Membrane-bound pyrophosphatases (M-PPases) are homodimeric primary ion pumps that couple the transport of Na+- and/or H+ across membranes to the hydrolysis of pyrophosphate. M-PPases are large (66–89 kDa), single-domain integral membrane proteins comprised of two identical monomers, each with 15–17 transmembrane helices. The helices of each subunit arrange into an inner ring (helices 5, 6, 11, 12, 15, 16) containing the functional core (active site, coupling funnel, ion gate, exit channel) and an outer ring (helices 1–4, 7–10, 13, 14) of largely unknown function. To date, H+-pumping (H+-PPase), Na+-pumping (Na+-PPase) and dual-pumping (Na+,H+-PPase) M-PPases have been found, most of which require potassium (K+) for maximal catalytic activity.

Following the inspection of enzyme key regions and structural alignments, it became clear that all of the data from 0 to 60 s could be combined into one, yielding a grouped structure of TmPPase in the resting state that is essentially identical to the individual 0-s (r.m.s.d./Cα: 0.33 Å) and TmPPase:CaMg (r.m.s.d./Cα: 0.29 Å) structure. The structure was solved at 2.54 Å along h, 2.95 Å along k and 3.38 Å along l with improved B-factors (108.65–70.28 Å2) and Rwork/Rfree values (21.95/23.61%) as compared to the 0-s structure (23.81/27.40%). The improvement in data quality parameters also translated into better electron density maps, so we could model most side chains and build additional key loop regions, for example, loop. Despite the presence of PPi in the crystallisation condition, it was not located at the active site, nor did it bind anywhere else. There were no observable significant changes in other regions of the protein, but the semi-conserved glutamate E6.53 appears to be flexible in all the structures as indicated by the absence of 2mFo-dFc density, even in the high-resolution 0–60 s structure, or negative density when modelled as seen in TmPPase:CaMg (Fig. EV3C). Ion binding is the first event, as there is no evidence of PPi in any of the structures before 60 s post Na+-addition, nor in the grouped 0–60-s structure, and the ion gate E6.53 appears disordered (Fig. EV3B): Na+ binding precedes substrate binding. Our TmPPase structure obtained in the absence of Na+ (0–60-s structure) suggests that in low Na+ conditions, E6.53 is not tightly coordinated at the ion gate, allowing it to loosely interact with S5.43. This could thus explain why K+-dependent Na+-PPases can pump protons at Na+ concentrations <5 mM.

>[2x]MRGSHHHHHHYVAALFFLIPLVALGFAAANFAAVVRKPEGTERMKEISSYIRSGADSFLAHETKAIFKVAIVIAILLMIFTTWQTGVAFLLGAVMSASAGIVGMKMATRANVRVAEAARTTKKIGPALKVAYQGGSVMGLSVGGFALLGLVLVYLIFGKWMGQVDNLNIYTNWLGINFVPFAMTVSGYALGCSIIAMFDRVGGGVYTKAADMAADLVGKTELNLPEDDPRNPATIADNVGDNVGDVAGLGADLLESFVGAIVSSIILASYMFPIYVQKIGENLVHQVPKETIQALISYPIFFALVGLGCSMLGILYVIVKKPSDNPQRELNISLWTSALLTVVLTAFLTYFYLKDLQGLDVLGFRFGAISPWFSAIIGIFSGILIGFWAEYYTSYRYKPTQFLGKSSIEGTGMVISNGLSLGMKSVFPPTLTLVLGILFADYFAGLYGVAIAALGMLSFVATSVSVDSYGPIADNAGGISEMCELDPEVRKITDHLDAVGNTTAAIGKGFAIGSAIFAALSLFASYMFSQISPSDIGKPPSLVLLLNMLDARVIAGALLGAAITYYFSGYLISAVTKAAMKMVDEIRRQAREIPGLLEGKAKPDYNRCIEITSDNALKQMGYPAFIAILTPLVTGFLLGAEFVGGVLIGTVLSGAMLAILTANSGGAWDNAKKYLEAGNLEGYGKGSEPHKALVIGDTVGDPLKDTVGPSLDILIKIMSVVSVIAVSIFKHVHLF>GTAELDALWNLVEAQYPVQTAAVTTLVTVPDDYKF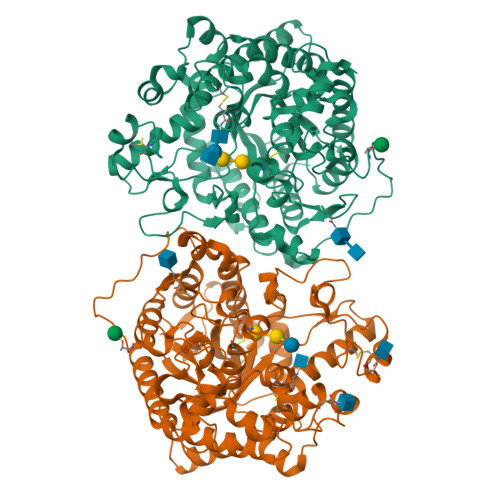EADPPSYALAGYETSEIAGLKFPKGFKFGVAGAAIQVEGAAKAEGRGPSTWDYLCHHYASTQCNNYDPDITTNHYYLYPLDFARLQHLGINTYSFSISWTRIYPLGAGYVNEAGLAHYDAVIHSAKKYGLEPVGTVFHWDTPLSLMLKYGAWQDTGDQIVKDFVTYATTVFKRYGNEVKTWFTFNEPRVFCSQNSGLPYNLTYPEGINSTSAVFRCTYNVLKAHGHAVKVYRDLVASGTIAAGEIGFKSDDNYPIPARPGNADDEESAKRHEAFRIGIFAQPVYGNGDYPDVVKETVGDMLPALTDEDKGYIKGSGDIFAIDGYRTDISHAALNGIANCIRNQSDPNWPVCEEGSDPFAHVYPSGFAIGQSADPLSSWLVNSAPFIRDQLKFLTQTYPAKGGIYFSAFGWAEDAEYDRQLLYQITWDGLRTQYLTDYLSQLLLAVHKDGINLRGALTWSFVDNWEWGLGMQQKFGFQFVNQSDPDLTRTFKLSAHAYAQFGRNHLHH[2x]>[3x]MITVDITVNDEGKVTDVIMDGHADH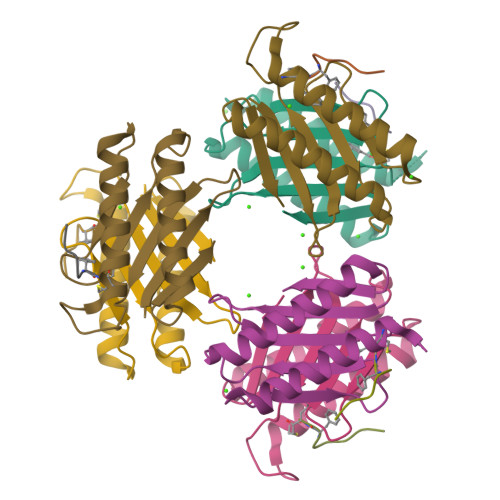GEYGHDIVCAGASAVLFGSVNAIIGLTSERPDINYDDNGGHFHIRSVDTNNDEAQLILQTMLVSLQTIEEEYNENIRLNYK;>KLNLQFF[3x]> DQWLQV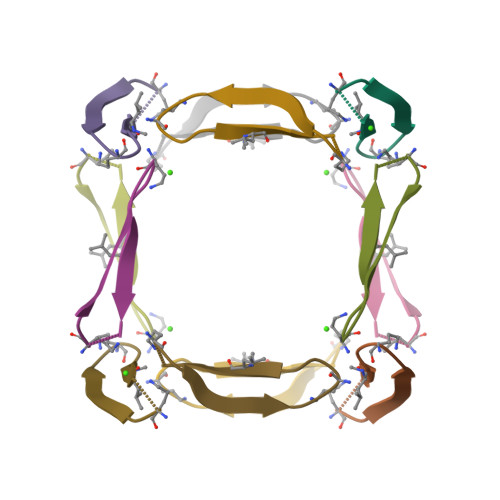DAEVTGIITA> MGEKRKTRQAEVNIGMVGHVDHGKTTLTKALTGVWTDTHSEELRRGITIKIGFADAEIRRCSNCGRYSTSPICPYCGHETEFIRRVSFIDSPGHEALMTTMLAGASLMDGAILVIAANEPCPRPQTREHLMALQIIGQKNIIIAQNKIELVDKEKALENYRQIKEFIKGTVAENAPIIPISALHGANIDVLVKAIEEFIPTPKRDSNKPPKMLVLRSFDVNKPGTPPEKLVGGVLDGSIVQGKLKVGDEIEIRPGVPYEEHGRIKYEPITTEIVSLQAGGQFVEEAYPGGLVGIGTKLDPYLTKGDLMAGNVVGKPGKLPPVWTDL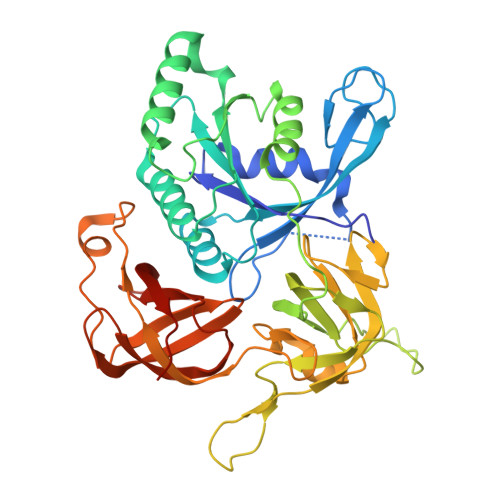RLEVHLLERVVGTEQELNVEPIKRKEVLLLNVGTARTMGLVTALGKDEIELKLQIPVCAEPGERVAISRQIGSRWRLIGYGIIKELEHHHHHH> AQLHSTVRAVPGNEN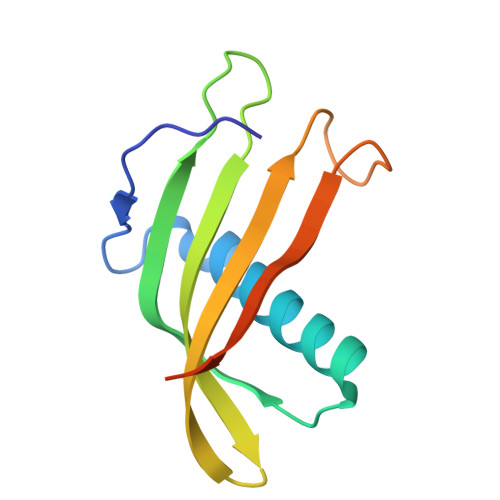SLEIEELARFAVDEHNKKENALLEFVRVVKAKEQYEDEHWFPGTMYYLTLEAKDGGKKKLYEAKVWVKNTAAPPSHMNFKELQEFKPVGDAAAAHHHHHH>MKKTKIVCTIGPKTESEEMLAKMLDAGMNVMRLNFSHGDYAEHGQRIQNLRNVMSKTGKTAAILLDTKGPEIRTMKLEGGNDVSLKAGQTFTFTTDKSVIGNSEMVAVTYEGFTTDLSVGNTVLVDDGLIGMEVTAIEGNKVICKVLNNGDLGENKGVNLPGVSIALPALAEKDKQDLIFGCEQGVDFVAASFIRKRSDVIEIREHLKAHGGENIHIISKIENQEGLNNFDEILEASDGIMVARGDLGVEIPVEEVIFAQKMMIEKCIRARKVVITATQMLDSMIKNPRPTRAEAGDVANTILDGTDAVMLSGESAKG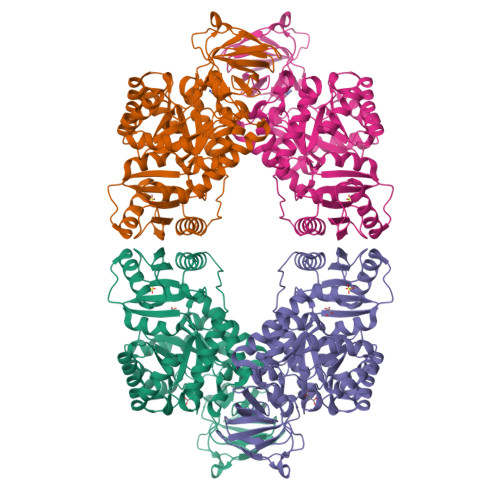KYPLEAVSIMATICERTDRVMNSRLEFNNDNRKLRITEAVCRGAVETAEKLDAPLIVVATQGGKSARAVRKYFPDATILALTTNEKTAHQLVLSKGVVPQLVKEITSTDDFYRLGKELALQSGLAHKGDVVVMVSGALVPSGTTNTASVHVL[2x]>AQVINTFDGVADYLQTYHKLPDNYITKSEAQALGWVASKGNLADVAPGKSIGGDIFSNREGKLPGKSGRTWREADINYTSGFRNSDRILYSSNWLI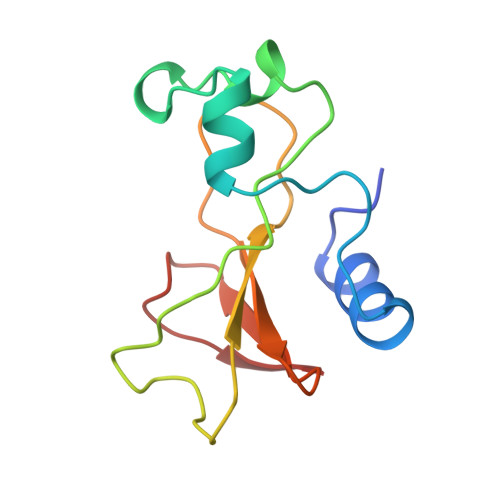YKTTDHYQTFTKIR[3x]>MVKLTLYGLDPSPPVRAVKLTLAALNLTYEYVNVDIVARAQLSPEYLEKNPQHTVPTLEDDGHYIWDSHAIIAYLVSKYADSDALYPKDPLKRAVVDQRLHFESGVVFANGIRSISKSVLFQGQTKVPKERYDAIIEIYDFVETFLKGQDYIAGNQLTIADFSLVSSVASLEAFVALDTTKYPRIGAWIKKLEQLPYYEEANGKGVRQLVAIFKKTNFTF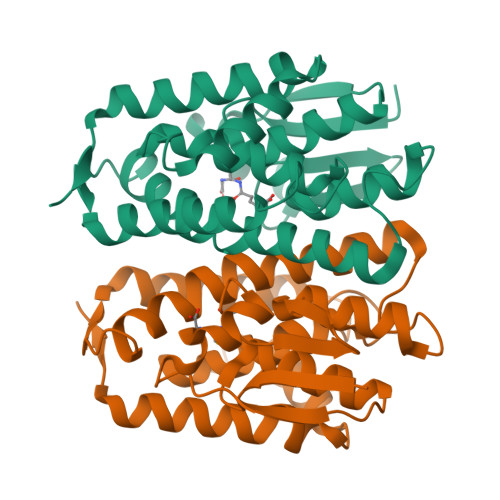EA[4x]> MLLVKAVKVLVMGGCMLPIAFGALGTGVLFAGFNVALSRNPEETESLFNNTLMGFALIETFIFMSIGLGFFVLFA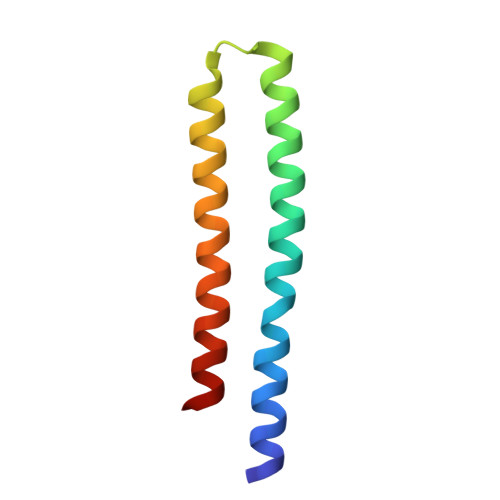A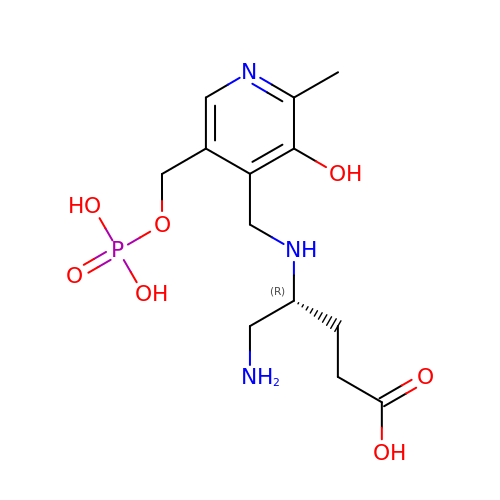(4R)-5-AMINO-4-[({3-HYDROXY-2-METHYL-5-[(PHOSPHONOOXY)METHYL]PYRIDIN-4-YL}METHYL)AMINO]PENTANOIC ACID | C13 H22 N3 O7 P | WQZRTAINNZJAQI-SNVBAGLBSA-N> MHHHHHHHHHHSGQNLYFQGHMATFISVQLKKTSEVDLAKPLVKFIQQTYPSGGEEQAQYCRAAEELSKLRRAAVGRPLDKHEGALETLLRYYDQICSIEPKFPFSENQICLTFTWKDAFDKGSLFGGSVKLALASLGYEKSCVLFNCAALASQIAAEQNLDNDEGLKIAAKHYQFASGAFLHIKETVL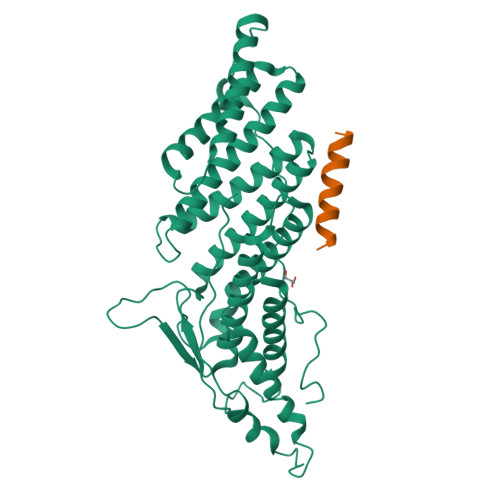SALSREPTVDISPDTVGTLSLIMLAQAQEVFFLKATRDKMKDAIIAKLANQAADYFGDAFKQCQYKDTLPKEVFPVLAAKHCIMQANAEYHQSILAKQQKKFGEEIARLQHAAELIKTVASRYDEYVNVKDFSDKINRALAAAKKDNDFIYHDRVPDLKDLDPIGKATLVKSTPVNVPISQKFTDLFEKMV;> KEEEDDDMKELENWAGSM> QTGSAPNHPSDSADSEYITSVSIGTPAQVLPLDFDTGSSDLWVFSSETPKSSATGHAIYTPSKSSTSKKVSGASWSISYGDGSSSSGDVYTDKVTIGGFSVNTQGVESATRVSTEFVQDTVISGLVGLAFDSGNQVRPHPQKTWFSNAASSLAEPLFTADLRHGQNGSYNFGYIDTSVAKGPVAYTPVDNSQGFWEFTASGYSVGGGKLNRNSIDGIADTGTTLLLLDDNVVDAYYANVQSAQYDNQQEGVVFDCDEDLPSFSFGVGSSTITIPGDLLNLTPLEEGSSTCFGGLQSSSGIGINIFGDVALKAALVVFDLGNERLG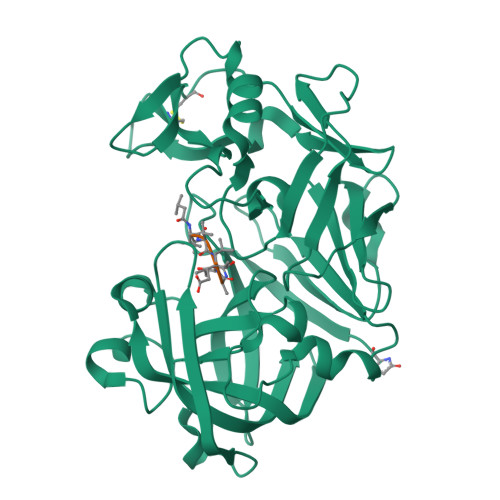WAQK>MTTAISAGTLPKEYQDLRDTVADFARSVVAPVSAKHDEEHSFPYEVVAKMGEMGLFGLPFPEEYGGMGGDYFALALALEELGKVDQSVAITLEAGVGLGAMPIYRFGNEEQKSKWLPDLLAGRALAGFGLTEPGAGSDAGSTRTTARLDGGEWVVNGSKQFITNSGTDITSLVTITAVTGSIADGKKEISTIIVPSGTPGFIVEPVYNKVGWNASDTHPLSFDDARVPEENLLGIRGKGYANFLSILDEGRIAIAALATGVAQGCVDESVKYAKERQSFGQPIGSYQAISFKIARMEARAHVARTAYYEAAAKMLAGKPFKK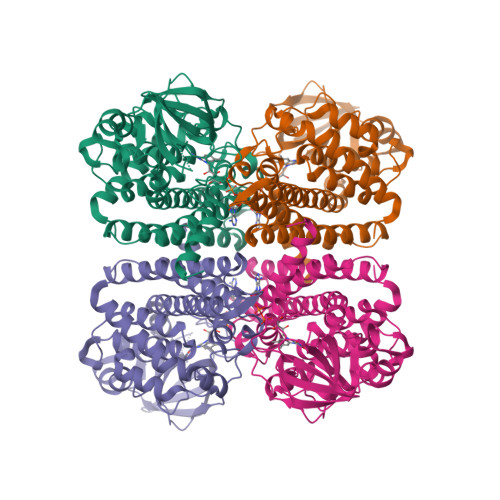EAAIAKMISSEAAMDNARDATQVHGGYGFMNEYPVARHYRDSKILEIGEGTTEVQLMLIARSLGLS[2x]> MASMTGGQQMGRDPSQVVQVNDSMYGFIGTDVVLHCSFANPLPSVKITQVTWQKSTNGSKQNVAIYNPSMGVSVLAPYRERVEFLRPSFTDGTIRLSRLELEDEGVYICEFATFPTGNRESQLNLTVMAKPTNWIEGTQAVLRAKK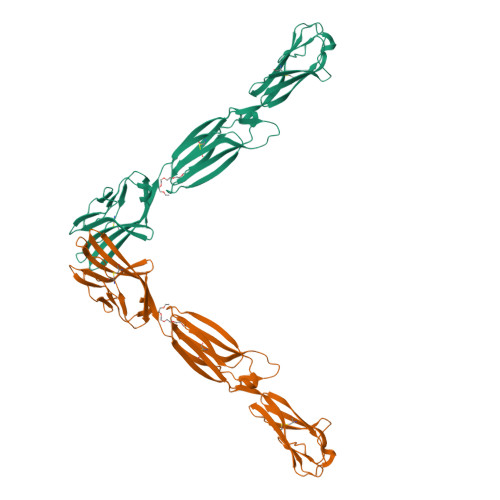GQDDKVLVATCTSANGKPPSVVSWETRLKGEAEYQEIRNPNGTVTVISRYRLVPSREAHQQSLACIVNYHMDRFKESLTLNVQYEPEVTIEGFDGNWYLQRMDVKLTCKADANPPATEYHWTTLNGSLPKGVEAQNRTLFFKGPINYSLAGTYICEATNPIGTRSGQVEVNITEAAALEHHHHHH> GPLGSKISKRVNAIEEVNNNVKLLTEMVMSHSQGGAAAGSSEDLMKELYQRCERMRPTLFRLASDTEDNDEALAEILQANDNLTQVINLYKQLVRGEE;>MAETRDQVKKLQLMLRQANDQLEKTMKDKQELE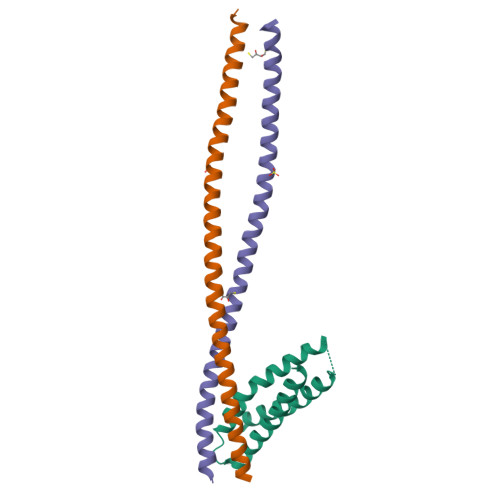DFIKQSSEDSSHQISALVLRAQASEILLEELQQGLSQAKRDVQEQMAVLMQSREQVSEELVRLQKDNDSLQGKHSLHVS[2x]> QEAQTELPQARISCPEGTNAYRSYCYYFNEDRETWVDADLYCQNMNSG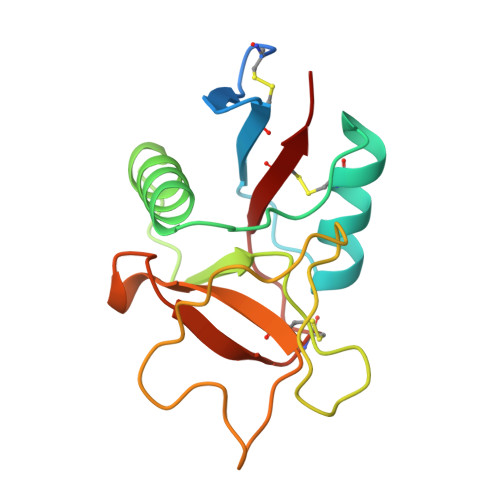NLVSVLTQAEGAFVASLIKESGTDDFNVWIGLHDPKKNRRWHWSSGSLVSYKSWGIGAPSSVNPGYCVSLTSSTGFQKWKDVPCEDKFSFVCKFKN> IVGGQECKDGECPWQALLINEENEGFCGGTILSEFYILTAAHCLYQAKRFKVRVGDRNTEQEEGGEAVHEVEVVIKHNRFTKETYDFDIAVLRLKTPITFRMNVAPACLPERDWAESTLMTQKTGIVSGFGRTHEKGRQSTRLKMLEVPYVDR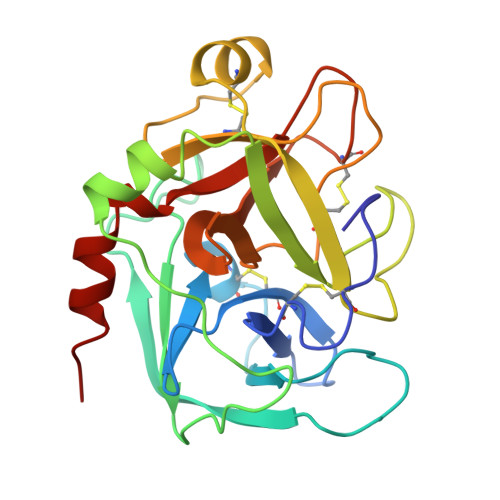NSCKLSSSFIITQNMFCAGYDTKQEDACQGDSGGPHVTRFKDTYFVTGIVSWGEGCARKGKYGIYTKVTAFLKWIDRSMKTR> MGGGGGGALNKLFPGYKDKIWMKVPVQWRQQMIQHWNKSYEKQVYSESVALNRTFQARNQLVLDRLKPSGAYRLPAVDYKRQLSRGTLVEGADFYLPTAQEQQRLARHFEPYSEQEQEERRKFRFQSISVYLAVALGASFVHDYFYQRRPVAWCLEKEPPH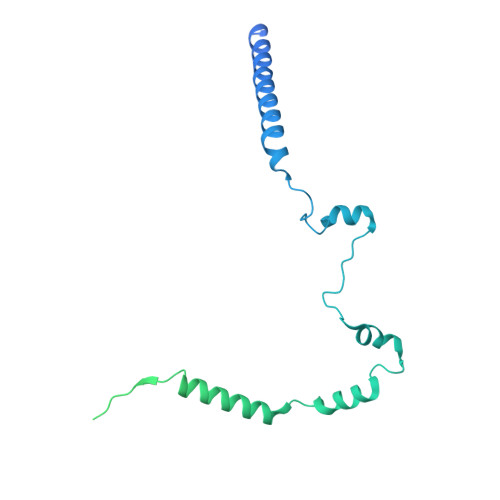PPSYPFWFKSLFHSHDIPSVRRGYEVYRKVCATCHSMEQLHFRHLVGEVLPEKRVKQIAAEYDVTDGPNDQGEMYTRPGILGDAFPSPYPNEEAARYANGGAYPPDLSLITAARHFGPDYLMALLGGYRDPPEGVELRPGLYWNVWFPGNAIAMPPPLMDEMIDYEDGTPCNISQMSKDVVNFLTWATEPTADERKLYGLKCVSAIAIGTVLMTLWWRFYWAMYATRRIDFGKLKYL> AAAAAAAA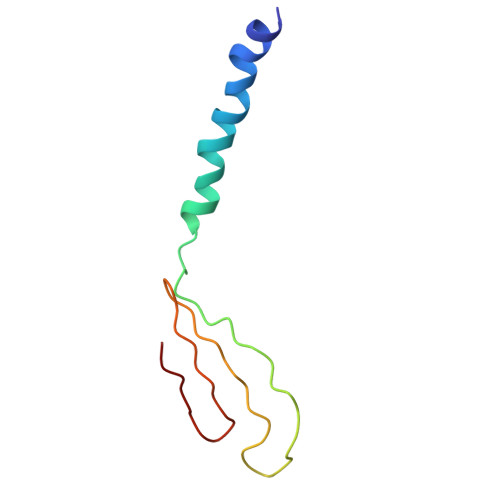AAAAAAAAAAAAAAAAAAAAAAAAAAAAAAAAAAAAAAAAAAAAAAAAAAAAAAAAAAAAAAAAAAA>MEEPDANGYYYHDTFEGSVGQWTARGPAEVLLSGRTAYKGSESLLVRNRTAAWNGAQRALNPRTFVPG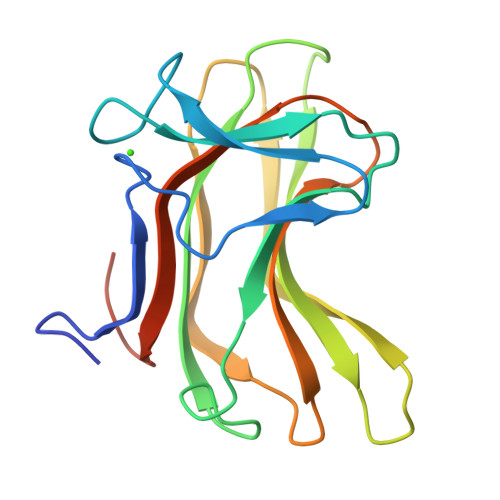NTYCFSVVASFIEGASSTTFCMKLQYVDGSGTQRYDTIDMKTVGPNQWVHLYNPQYRIPSDATDMYVYVATADDTINFYIDEAIGAVAGTVIEGLEHHHHHH[2x]Hence, this loss of critical proteins has the potential to compromise ER proteostasis and generate cellular stress. This challenge to normal metabolism is overcome by the activity of the cytosolic coatomer protein I (COPI) polymer, whose repeating unit is the coatomer, a 560 kDa complex of seven distinct gene products (α-, β-, β′-, γ-, δ-, ε-, and ζ-COPI)25–31. Overall, the coatomer functions to retrieve the escaped “client” proteins, such as type I membrane proteins, from cis-Golgi back to ER by retrograde trafficking. In particular, the S protein – a type I membrane protein – is delivered to the ERGIC from both the ER (by anterograde trafficking) and the Golgi (by retrograde trafficking)3,10–12. Here we utilize recombinant SARS-CoV-2 S proteins and tail peptides, including constructs with enhanced mimicry of the coatomer binding motif (clientized S protein), to elucidate the atomic structure of the S-coatomer interface.

To gain insight into the role of the basic cluster in stabilizing S-coatomer interactions, we generated alanine mutants of αWD40 Arg13, Lys15, and Arg300, which are equivalent to the β‘WD40 basic cluster residues Arg15, Lys17, and Arg272, respectively. The αWD40 Arg300Ala mutation yielded similar dissociation constants (KD) of 3.6 ± 0.4 µM and 4.2 ± 0.4 µM for wild-type and clientized Thr1273Glu S heptapeptides, respectively, and a 1.8 Å resolution crystal structure showed minimal perturbation of the binding site in this β‘WD40 mutant. This suggests that the αWD40 Arg300 side chain is important for the higher affinity for the clientized S heptapeptide. I Superposition of wild-type (white) and Arg300Ala mutant (yellow) crystal structures shows minimal perturbation near the mutation site. Site-directed mutagenesis of this basic cluster showed that an arginine at position 300 in αWD40 determines this enhanced affinity.

>[3x]MEMLTKFESRSSRAKGVAFHPTQPWILTSLHNGRIQLWDYRMGTLLDRFDGHDGPVRGIAFHPTQPLFVSGGDDYKVNVWNYKSRKLLFSLCGHMDYVRVCTFHHEYPWILSCSDDQTIRIWNWQSRNCIAILTGHSHYVMCAAFHPSEDLIVSASLDQTVRVWDISGLRMKNAAPVSMSKEDQKAQAHNSKSNDKKGSTDAIVKFVLEGHDRGVNWCAFHPTLPLILSAGDDRLVKLWRMTASKAWEVDTCRGHFNNVSCCLFHPHQELILSASEDKTIRVWDLNRRTAVQTFRRDNDAFWFITVHPKLNLFAAAHDSGVMVFKLESAWSHPQFEK Omniligase-1 is a broadly applicable enzyme for peptide bond formation between an activated acyl donor peptide and a non-protected acyl acceptor peptide. The enzyme is derived from an earlier subtilisin variant called peptiligase by several rounds of protein engineering aimed at increasing synthetic yields and substrate range. Mutation A225N in the S1′ pocket and F189W of the S2′ pocket increased the synthesis to hydrolysis (S/H) ratio and overall coupling efficiency, whereas the I107V mutation was added to S4 pocket to increase the reaction rate. The final omniligase variants appeared to have a very broad substrate range, coupling more than 250 peptides in a 400-member library of acyl acceptors, as indicated by a high-throughput FRET assay.

In comparison to the Pre-1 and Pre-2 variants, Pre-3 has the additional mutation A225N at the S1′ pocket that is also present in Oml-1. This remarkable A225N mutation almost doubles the S/H ratio (see above), which asks for a structural explanation. The sidechain of Asn225 in the α-helix close to the active site has a hydrogen bond to the hydroxyl group of Ser125 providing a more restrained position than in Pre-1 or Pre-2. Furthermore, Asn225 has H-bonds to the sidechain of Asn123 and the carbonyl oxygen of the non-oxidized Cys221, and thus makes good contacts, possibly rigidifying, with the local active site environment of omniligase-1. The S1′ pocket becomes shallower by ca. 2.5 Å but about 1.3 Å wider compared to variants Pre-1 and Pre-2, providing even less steric crowding (see above). The asparagine side chain is larger than that of a proline, but points in a different direction; it is located between the α-helices that the catalytic triad residues Cys221 and His64 are positioned upon and as a result these residues are pushed away from each other. The Cα-Cα distances increase by 0.4 Å for residue 225 and Val68 and by approximately 1 Å for Cys221 and His64. In summary, the A225N mutation could improve the S/H ratio by shortening the Cys221 helix in the same way as the P225A mutation, creating space for the cysteine. The A225N substitution also widens the S1′ binding pocket by pushing His64 and Cys221 apart, which is facilitated by formation of H-bonds to nearby residues and to two water molecules in the S1′ pocket.

> AKCVSYGVSQIKAPALHSQGYTGSNVKVAVIDSGIDSSHPDLNVAGGASFVPSETNPFQDNNSHGTHVAGTVLAVAPSASLYAVKVLGADGSGQYSWIINGIEWAIANNMDVINMSLGGPSGSAALKAAVDKAVASGVVVVAAAGNSGTSGSSSTVSYPAKYPSVIAVGAVDSSNQRAPFSSVGPELDVMAPGVSICSTLPGNKYGAHSGTCPASNHVAGAAALILSKHPNWTNTQVRSSLENTATKLGDSFYYGKGLINVEAAAQHHHHHH> GSPGIRLGSSEDNFARFVCKNNGVLFENQLLQIGLKSEFRQNLGRMFIFYGNKTSTQFLNFTPTLICADDLQTNLNLQTKPVDPTVDGGAQVQQVVNIECISDFTEAPVLNIQF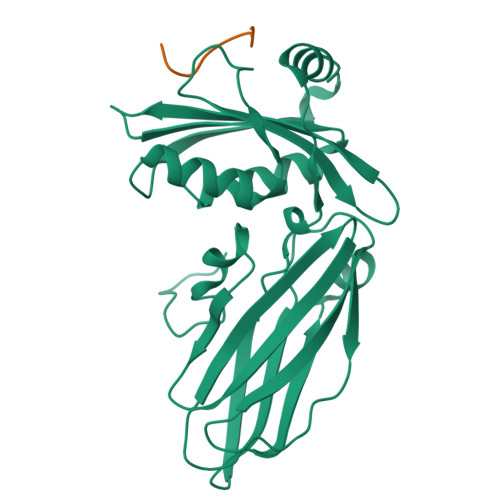RYGGTFQNVSVKLPITLNKFFQPTEMASQDFFQRWKQLSNPQQEVQNIFKAKHPMDTEITKAKIIGFGSALLEEVDPNPANFVGAGIIHTKTTQIGCLLRLEPNLQAQMYRLTLRTSKDTVSQRLCELLSEQF;> SFFEDNFVPE>[2x]GMDKLTHYRHTIQEIIKKYYDLSNSQPATATETKISDDLPDTVGDRLIIDEQ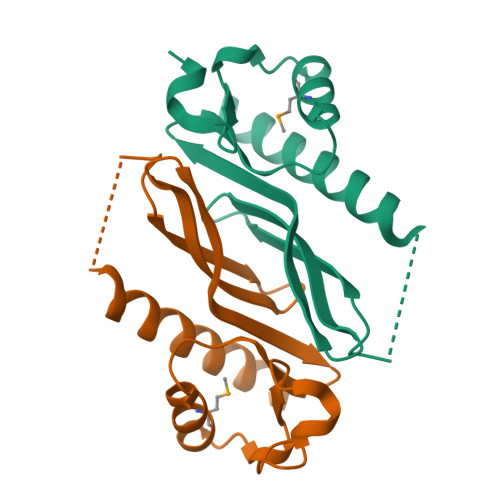RDQYLWLCCGWDGKKRVQHIILYLQIQNGKIWIEEDSTNLAIVDEMLVAGIPQTDIILGFHHPSKRGLTEFAIA> 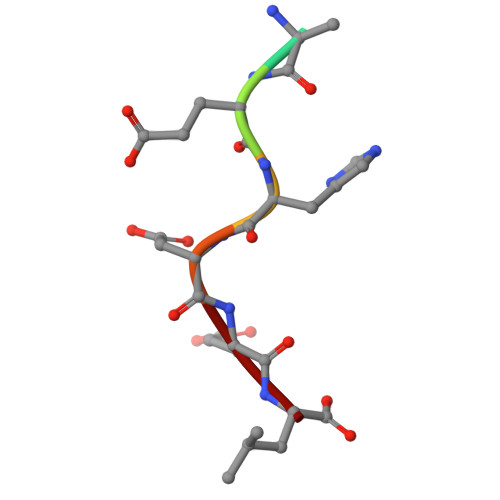TAEHDEL> ADRHTVFWNSSNPKFRNEDYTIHVQ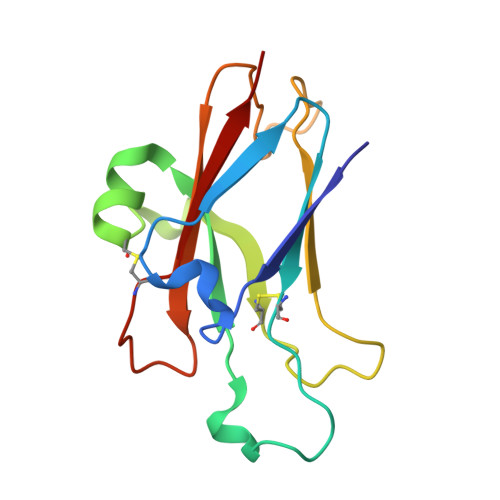LNDYVDIICPHYEDHSVADAAMEQYILYLVEHEEYQLCQPQSKDQVRWQCNRPSAKHGPEKLSEKFQRFTPFTLGKEFKEGHSYYYISKPIHQHEDRCLRLKVTVKI(E)-2-(5-CHLOROTHIOPHEN-2-YL)-N-[(3S)-1-{4-[(1S)-1-(DIMETHYLAMINO)ETHYL]-2-FLUOROPHENYL}-2-OXOPYRROLIDIN-3-YL]ETHENESULFONAMIDE 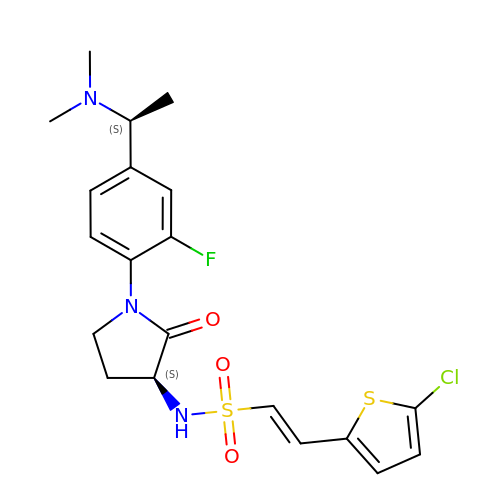| C20 H23 Cl F N3 O3 S2 | AFDHTIFDRFSZDA-WZMLOTFKSA-N> GGGGGACGGUCCGGCGACCAGCGGGUCUCUAAAACCUAGCCAGCGGGGUUCGACGCCCCGGUCUCUCGCCA

Pyrrolysyl-tRNA synthetases (PylRSs) are naturally encoded in some archaeal and bacterial genomes to acylate tRNAPyl with pyrrolysine. Similar to the 20 canonical amino acids, Pyl also has a dedicated tRNA:aaRS pair (tRNAPyl:PylRS) for protein translation. To reveal the mechanism by which the Ma tRNAPyl identity elements mediate highly specific recognition of Ma tRNAPyl by MaPylRS, we determined two cryo-EM structures. We achieved high resolution (2.8–2.9Å) maps by using the ribosome as a scaffold for visualizing Ma or Mm tRNAPyl, a strategy that we previously showed to be successful.

Comparison of these two structures revealed four unique structural features of Ma tRNAPyl compared to Mm tRNAPyl, providing insight into its orthogonal recognition by MaPylRS. The first major difference is the absence of a base at position 8 (at the acceptor/D-stem junction). This missing base causes changes in the overall structure of the linker between the acceptor stem and the D-stem. In Mm tRNAPyl, as in other tRNAs, the presence of U8 pushes G10 into a loop. However in its absence (Ma tRNAPyl), G10 resides right next to C7, resulting in an atypical conformation of bases C7 and G10. A second difference is the A42a-bulge, named for its appearance as a bulge in the Ma tRNAPyl secondary structure due to its inability to base-pair with either C27 or G28 in the anticodon stem. Our tertiary structure reveals that this bulge is not visually present. Instead, A42a is sandwiched between two base pairs, C27:G43 and G28:U42. As an apparent consequence of this intercalation of A42a into the acceptor stem of the tRNA molecule, we observed an upward shift of nucleotides 43 and 44 towards the acceptor stem, altering the tRNA structure. However, the two tRNA structures began to deviate from each other (rmsd ∼1.5 Å between their backbone atoms) within a stretch between U8 and U28 in Mm tRNAPyl. This overall shape change appears to be caused by the elements in Ma tRNAPyl which we determined to be necessary for MaPylRS recognition; the deletion of U8 in Ma tRNAPyl truncating the loop between the acceptor stem and D-stem, and the mutation of U28:G42 to G28:U42 (and possibly the A42a intercalation) affecting the trajectory of the phosphate backbone.>[4x]GSNNSETPAPGPDSLLALAFPSDPQVSPDGKQVAFVLAQISEEDPAKPDKDFARPRYRSGLWLSEGGAARPLTHAETGRGDSAPRWSPDGQNLAFVRSAGEVKAALMLLPLKGGEARRVTHFKNGVSGPQWSPDGRFIAFTTTADTEDKRDERGEARVLTRPVYRANGADWLPERPAALWLYDVEADKLREWYAPEIGI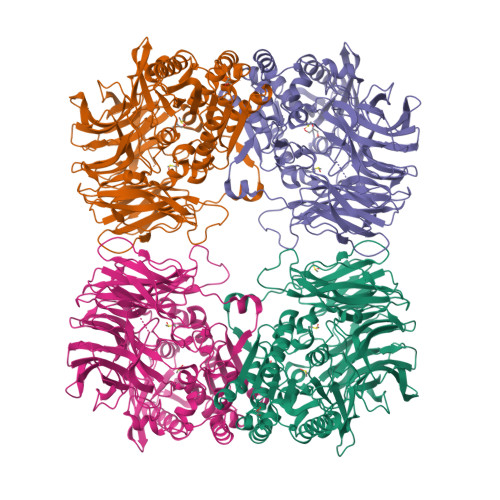GALSWWPDSRGVLIVQSEDEWQASQWRQDVYDLPLPTADAPAAPQKLLDWNSAAHGLAPHPDGQRFALIGRPAGKGNTEHAHLYLIENGQHRRLDTGHDHPVGDAVGGDCHVGAFPEGPRWLDGDTLLFSSTVRGSVGLFTAHIGGGVKAYDHDPQGVISAFTANEHGVALIRESATRFPEVELNGQRVTDLHARFPFPVREPQRVTFETELGEGEGWVLLPEGEQKVPALLNIHGGPHTDYGHGFTHEFQLMAARGYGVCYSNPRGSVGYGQAWVDAIYGRWGTVDADDLLNFFDRCLEAVPRLDAAKTAVMGGAYGGFMTNWITGHTTRFQAAITDRCISNLISFGGTSDIGLRFWDDELGLDFSRRADALKLWDLSPLQYVENVKTPTLIVHSVLDHRCPVEQAEQWYAALHKHQVPVRFVRFPEENHELSRSGRPDRRLTRLNEYFAWLERWL>MAARDPEATKARIFEAAVAEFARHGIAGARIDRIAAEARANKQLIYAYYGNKGELFASVLEKKMLDLAISVPVDPDDIEGWIDRLLDYHAAHPELLRLLFWEGMEYGTAELPHEAERQEHYARKVAAVRDGQERGVITDAIPAPDLLFLLVAMANWAVVVPQMK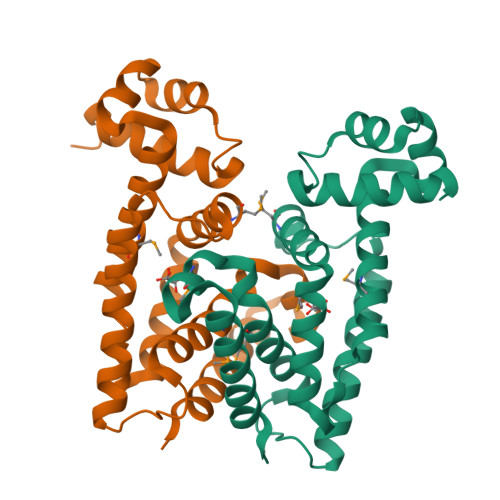RILVGGGDAGTDGLRDSIKKAARRIVDRRSLEHHHHHH[2x]>[6x]MAGNETIETF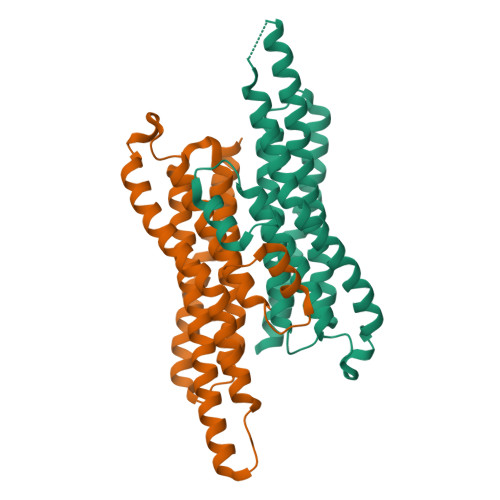LDGLASSAPTPGGGGAAAISGAMGAALVSMVCNLTIGKKKYVEVEADLKQVLEKSEGLRRTLTGMIADDVEAFDAVMGAYGLPKNTDEEKAARAAKIQEALKTATDVPLACCRVCREVIDLAEIVAEKGNLNVISDAGVAVLSAYAGLRSAALNVYVNAKGLDDRAFAEERLKELEGLLAEAGALNERIYETVKSKVNLEHHHHHH> MQNLEAQVTGSLVAFPDVTQKALKEDEINLDSVLRGKFSTGRTSLAWLACGPQLEITNSVTGERISAYHFSGLTERPPVVVAVKEFTWQKKTGLLVGLVEAEGSVLCLYDIGISKVVKAVVLPGSVTAVEPIINHGGASASTQHLHQSLRWFFGVTAVVTDVGHVLLIDLCLDEVSSNQDELDASDLEVMSVIPTKIPKLREAATRERRHLCLQLAAPTGTTVSCLSYISRTNQLAVGYSDGYFSLWNMKTLRRDYHVQIEGGRVPVCAVAFQEPENDPRNCCYLWAVQSSESGGDVSLHLLQLAFSDRKCLASGQIMYELLEYCEERYSLDLSGSTLSLRGQSNNTKLLGCQTIEKFRVHGEREDGVHEVTSPDTSVSVFSWQVNTYGQGKPSVYLGVFDINRWYQAQMPDSLRSGQFLRNCSYFAFWSLEAVVNITTQDIIFDILVHERSLSRGIPPSYPPPEQFYYPSTYNFDATCLLNSGLIHFACTGFQKETLHFLKKSGSSLNEAIPDGYNRCLAAGLLAPKFTDVQASSLSQEEQLQAILAAAVETSSLGLLTSCIKRWTAEEQPRSAANLRFVLEWTWKKVTLTKQEFDRLCFRLFDGSCNFIDPHTLQSLQQCHLYFSNLTAVLNCFIAQAKEVTQQGAVDLTNKQSVTRLLTLYASVVLWFCRSGMLPDSSDETVQLTRPFYNYQVIQQYYSDQRKKLERLARGKWDTSSLMIDGLINQFGDRIQQLWSRDDNGTGKYPPANLHALLDVYLLENADEMSKHAITIYFLLDIMYSFPDKPDSSIESFPTAFFVPGSLIKLIQGFWLLDHNDYQNSVDCILNPASSRVMSWQHSQIIENLLCHGDSRQALRYLQVMKPVATTSKEVKLHMTVLLANRSILEAWNLQRLHSSRLNVEELLKHMYEMCQEMGLIEELLKLTFTDFEQGYLHKFLQTTGVQNQELLLVHHLQRANYISALQLNQSLKTNHLNDCDRRLRERSGARNAILDQYGKILPRVQRTLASERAKPYSLPSLVWREVARPKPLSTTAKQAAPGSIITKANFICNVLSKIKEVSTANEKREEYSPYQSMVSEEPTAPPLQDIDVPDAFFGTPINKSRRVSRLLDSVVHPVLMEPTPLTSSDTDNNQTPHKSPLLKTSSPLHSSLRRIAHMRSFAKASEFSLLETPLVVRKAKALAANTASSGYTSITPQSILRSSVRTTPLVSPSVSPGRSLTPPLRPKETKISFMELSFTRHAKAAHSSEGNLLAISPVLRSSPDAVWSVKGKVASFTQNTPVKKLDEIDASSSGIQEESQDEMEVSKEISNISVRSEQASLEYHDAPTPEDLENDEISGTTNSQPQVNEVHHQMEDGQLTEKPAELALTEMQEEFIDSEEREIEYISAPLNGPNALECMTAVPDIYLEDASQCILETPEGSSVSVT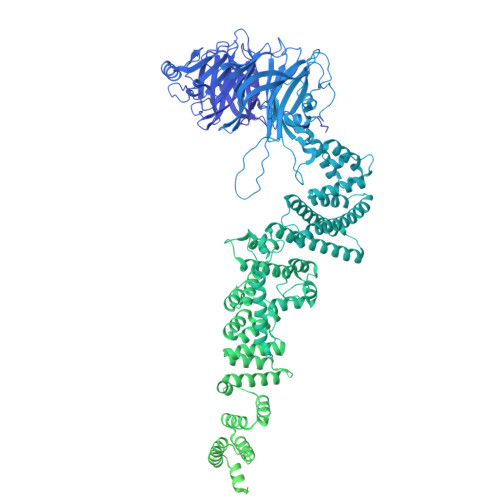GEQECVSSAKDSESVISIHDSDDAHSNLSENDQDSEEIEENNLRVPTTVTRCEEFDLIETKDLEVELEEADSEKTNYKDIYPDATVQLGFTVESIEQRYTCELADRRETPSETDEIEGEHFETENNFSLVLEGDVTEEEILEPSSSKTDLELTRPPIAHQKLISENRENIENCETTEKIPANMSPLVDSDHESKTLETLPSEADLSVAEKVLKGTEEKDVPPEVHSEVVLESKLVGNAMMSLDSSESQEVIISQYDNVISIEKLEMTQEKMYGEKTEQINEGQVSPNRDQSTLVKPLTPRRSIRKSSKPADSSTDIIGNITLPTTPKRGLKKAKENVDTLKNSISVVPEEELTLGTRRITRKATLTALDNPEPLQIKEPPSGEDLQVQPSTPTRGRRGKVITSDDLKEPPSGEDLQVQPSTPTRGRRGRVITSDDLREPPPGEDLQVQPSTPTRGRRGRVITSDDIKESPSVEDLQVQPSTPTRGRRGKVITSDDIKEPPSVEDLQVQPSTPTRGRKGKVITSDDIKEPLSGEDLQVQPSTPTRGRKGKVITSDDIKEPLSEEVLQEQPSTPTRGRRGRVITSDGKGYECVEEKNALPLTPTRITRSKNILEPEKGISQIEPEKGISQIEPDKGLSQIEDTGETEHEVVTPRRGRRGKRVVNELVKHFERNSSQPNIKADTSPPVSPKKVSLRWTRTRSENQRINATEEQASKIQEDLSDTPRKRYKKSSNKMGFEETTDTVTEGAIVEDVQESLIISHLGKNPNTSIVRSARKTALPPVTEDHSEQPLLPPESHSKVHSSLAIADEENKTNTRTRSGNKSSVDVSAITFEFSTPKARTKKTAKGSAVPTELIPSTQYVFSPPSTRTRRATRANVSEAVIEPQLQFQESCEIAETEVPEVPASKPRGRPPKHKAKAVTRVLKKPSWSTPPVEIKLISPPESPAVSETNTKTDSTEAKGAEKISVRRTRRRIIAKPVTRRKMR>[2x]SGSSLQQHLSNRDPRPLRDKNFQSAIQEEIY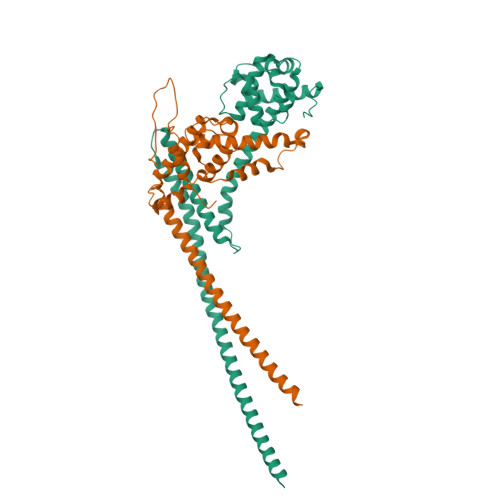DYLKKNKFDIETNHPISIKFLKQPTQKGFIIIFKWLYLRLDPGYGFTKSIENEIYQILKNLRYPFLESINKSQISAVGGSNWHKFLGMLHWMVRTNIKLDMCLNKVDRSLINQNTQEITILSQPLKTLDEQDQRQERYELMVEKLLIDYFTESYKSFLKLEDNYEPSMQELKLGFEKFVHIINTDVTSTELKLEELKVDLNRKRYKLHQQVIHVIDITSKFKINIQSSLENSENELGNVIEELRNLEFETEHNVTN;>MKLRRKSILHTIRNSIASGARISLGSGAARVVNGPVSRNQDVFPILDLQELVICLQSCDFALATQENISRPTSDYMVTLYKQIIENFMGISVESLLNSSNQETGDGHLQEENENIYLDTLNVLVLNKICFKFFENIGVQDFNMTDLYKPEAQRTQRLLSAVVNYARFREERMFDCNSFILQMESLLGQINKLNDEIKQLQKDFEVEVKEIEIEYSLLSGHINKYMNEMLEYMQ[2x]> HHHHHHGSMGFLILSRREGEGITLSLKADYPAEELIRQLREGGIRILVTDIIGNQARVGIEA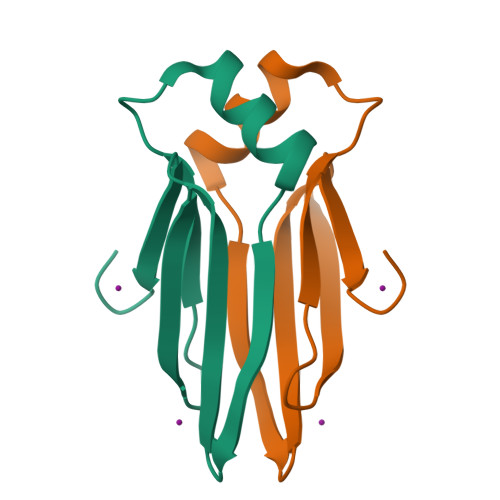PRGVLIVRDELKTAPKG>MNVASRVVVNADRVKGTINRNIYGHFSEHLGRCIYEGLWVGEDSPIPNTNGIRNDVLEALKQMKIPVLRWPGGCFADEYHWKDGVGPREKRKRMVNTHWGGVIENNHFGTHEFMMLCELLGCEPYISGNVGSGTVQEMSEWVEYITFDGESPMANWRRENGREKPWRIKYWGVGNQNWGCGGNMRAEYYADLYRQFQTYLRNYGDNKLHKIACGANTADYHWTEVLMKQAAPFMHGLSLHYYTVPGPWEKKGPATGFTTDEWWVTLKKALFMDRLVTKHSAIMDVYDPDKRIDLIVDEWGTWYDVEPGTNPGFLYQQNSIRDALVAGATLHIFHRHCDRVRMANIAQLVNVLQSVILTEGERMLLTPTYHVFNMFKVHQDAELLDTWESVERTGPEGELPKVSVSASRAADGKIHISLCNLDFETGASVDIELRGLNGGVSATGTTLTSGRIDGHNTFDEPERVKPAPFRDFKLEGGHLNASLPPMSVTVL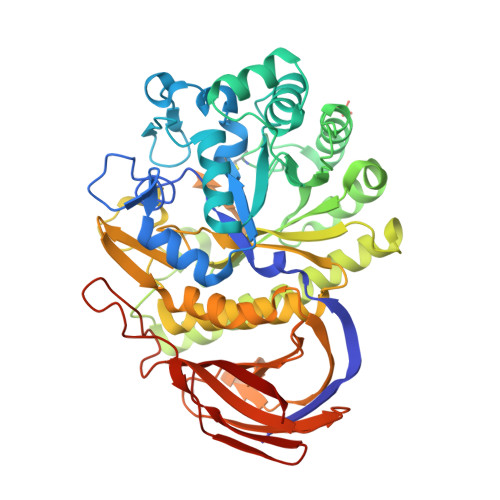ELTAG[3x]S. meliloti possesses two BolA-like proteins (BolA and YrbA), the function of which is unknown. In the present study, we have performed a structure–function analysis of SmYrbA showing that it coordinates diverse divalent metal ions (Fe2+, Co2+, Ni2+, Cu2+ and Zn2+) using His32 and His67 residues, that are also used for Fe–S cluster binding in BolA–Grx heterodimers. It also possesses the capacity to form heterodimers with the sole monothiol glutaredoxin (SmGrx2) present in this species. It shows a winged helix-turn-helix motif formed by four helices and a three-stranded β-sheet (α1β1β2η2α3α3′β3 in which η: 310-helix).

Suitable X-ray diffracting crystals were obtained in a crystallization solution containing nickel chloride. Thus, a MAD experiment was attempted at the absorption edge of the nickel atom (Z = 28). We successfully phased the 0.98 Å resolution data with one Ni atom per monomer. This first structure was named SmYrbA-Ni. The calculated low solvent rate of 37% could explain the high diffraction power of the crystals of SmYrbA–Ni and SmYrbA–Cu complexes. The Co, Cu and Ni metal ions are coordinated in an octahedral geometry, bound to His32 and His67 of SmYrbA and four water molecules. In SmYrbA–Co and SmYrbA–Ni structures, the metal atom is almost equidistant from its ligands with a metal–ligand distance of 2.3 and 2.1 Å, respectively. All these residues belong to the [H/C]-loop, but both Asp and Leu residues are not or poorly conserved in YrbA/BolA proteins.

> MAPGDIEDMIKAGIPGARVTIRDLAGDGDHYAAEVVAEAFRGKTRVQQHQMVYNALKGNMGGILHALALQTSAPE> MAHHHHHHMVNVAVIGAAGGIGQSLSLLLLRELPFGSTLSLYDVVGAPGVAADLSHIDRAGITVKHAAGKLPPVPRDPALTELAEGVDVFVIVAGVPRKPGMTRDDLFNVNAGIVMDLVLTCASVSPNACFCIVTNPVNSTTPIAAQTLRKIGVYNKNKLLGVSLLDGL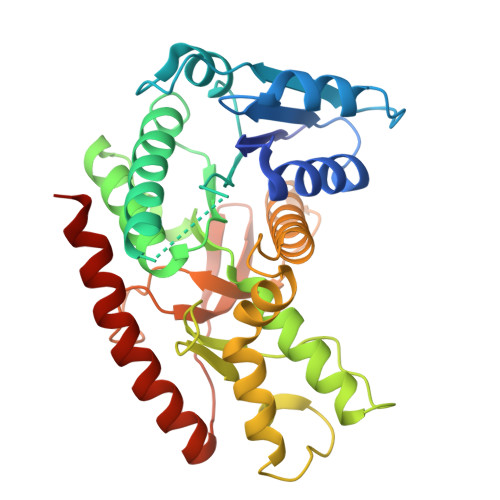RATRFINNARHPLVVPYVPVVGGHSDVTIVPLYSQIPGPLPDESTLKEIRKRVQVAGTEVVKAKAGRGSATLSMAEAGARFTMHVVKALMGLDTPMVYAYVDTDGEHECPFLAMPVVLGKNGIERRLPIGPITTVEKEMLEEAVGVVKKNIAKGETFARSKL1-cyclopentyl-6-[[(2R)-1-(2-oxa-6-azaspiro[3.3]heptan-6-yl)-1-oxidanylidene-propan-2-yl]amino]-5H-pyrazolo[3,4-d]pyrimidin-4-one | C18 H24 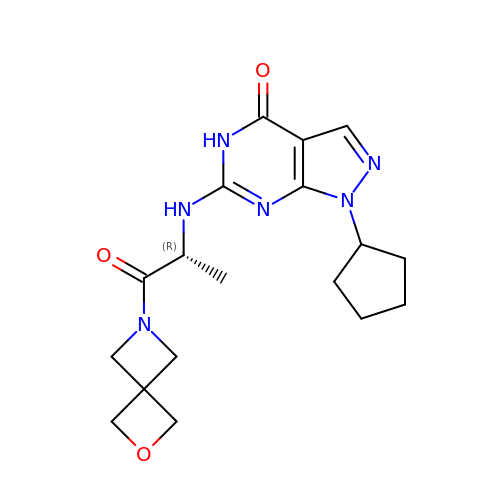N6 O3 | KCKFQVCSNMDMEM-LLVKDONJSA-N> MDSQRNLLVIALLFVSFMIWQAWEQDKNPQPQAQQTTQTTTTAAGSAADQGVPASGQGKLISVKTDVLDLTINTRGGDVEQALLPAYPKELNSTQPFQLLETSPQFIYQAQSGLTGRDGPDNPANGPRPLYNVEKDAYVLAEGQNELQVPMTYTDAAGNTFTKTFVLKRGDYAVNVNYNVQNAGEKPLEISSFGQLKQSITLPPHLDTGSSNFALHTFRGAAYSTPDEKYEKYKFDTIADNENLNISSKGGWVAMLQQYFATAWIPHNDGTNNFYTANLGNGIAAIGYKSQPVLVQPGQTGAMNSTLWVGPEIQDKMAAVAPHLDLTVDYGWLWFISQPLFKLLKWIHSFVGNWGFSIIIITFIVRGIMYPLTKAQYTSMAKMRMLQPKIQAMRERLGDDKQRISQEMMALYKAEKVNPLGGC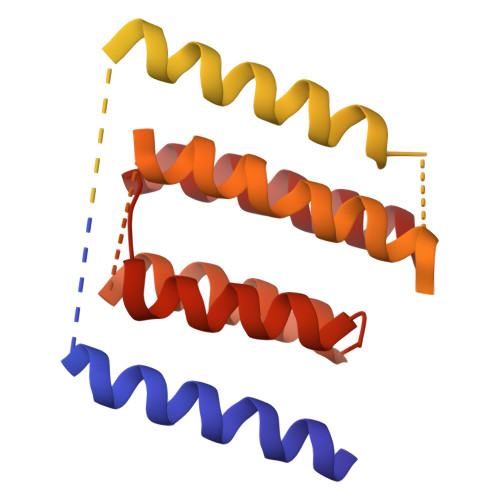FPLLIQMPIFLALYYMLMGSVELRQAPFALWIHDLSAQDPYYILPILMGVTMFFIQKMSPTTVTDPMQQKIMTFMPVIFTVFFLWFPSGLVLYYIVSNLVTIIQQQLIYRGLEKRGLHSREKKKS> MVLRKVVAILLAILPIFLFAVEPVVVVRSEKEIVVLTRFEEYHFDLEKGILKDFYTLVDGRKHVFTYGNDGFDVLDEGTPLTVIEEPIVTGVGKVSEGFSDEVSIVYNYGYVKKIFTIKNNENYTFFVDIESSKPVDVTVPRVSVDTSTDRYLENYFASFNPKTRTLVLLKHDEGLLFEGTLKVNGQKRFIVFMGPNKRTLIKKAFPEDYDVLIKALVNIPGFNKWYDSVFYGLVWFFWWLKDLTKNFGWAIMLFTLIVRLILYPLYHAQTKSLINMRKLQPQIEAIKKKYKDPTKQQEALLKLYREAGVNPASGCLMLLIQLPIFMLLWSVIRYYVEEFAYSGSFLIWKDLSAGGFSNNWLFLVITIVASYYTTLLTSQDARTAWQGIIMSVIFPFLFVGLPSGLFLYYATNTLIQLAVTYYT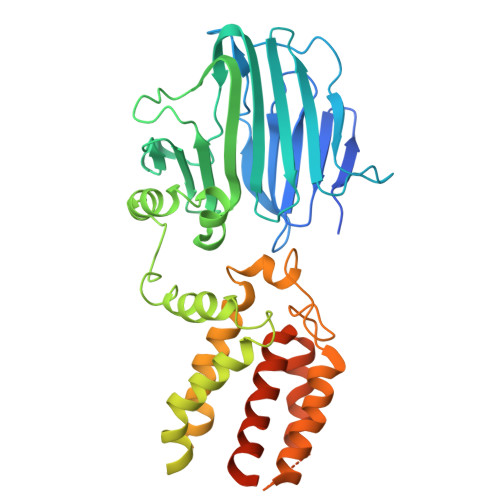YKRYKIKGLTTRELLGLPKKAHHHHHH>[2x]QKPGETKEVHPQLTTFRCTKRGGCKPATNFIVLDSLSHPIHRAEGLGPGGCGDWGNPPPKDVCPDVESCAKNCIMEGIP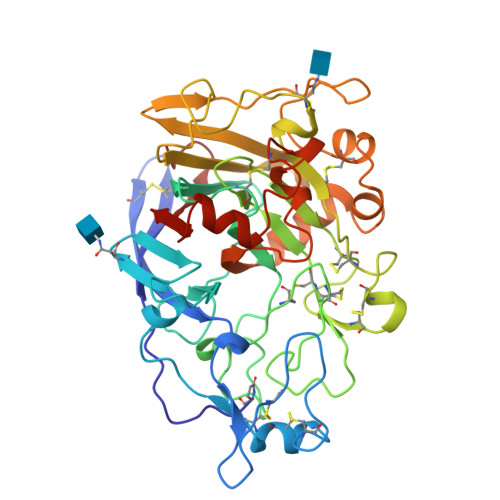DYSQYGVTTNGTSLRLQHILPDGRVPSPRVYLLDKTKRRYEMLHLTGFEFTFDVDATKLPCGMNSALYLSEMHPTGAKSKYNPGGAYYGTGYCDAQCFVTPFINGLGNIEGKGSCCNEMDIWEANSRASHVAPHTCNKKGLYLCEGEECAFEGVCDKNGCGWNNYRVNVTDYYGRGEEFKVNTLKPFTVVTQFLANRRGKLEKIHRFYVQDGKVIESFYTNKEGVPYTNMIDDEFCEATGSRKYMELGATQGMGEALTRGMVLAMSIWWDQGGNMEWLDHGEAGPCAKGEGAPSNIVQVEPFPEVTYTNLRWGEIGSTY> NVIQDLYLRELKDTKLAPSTLQD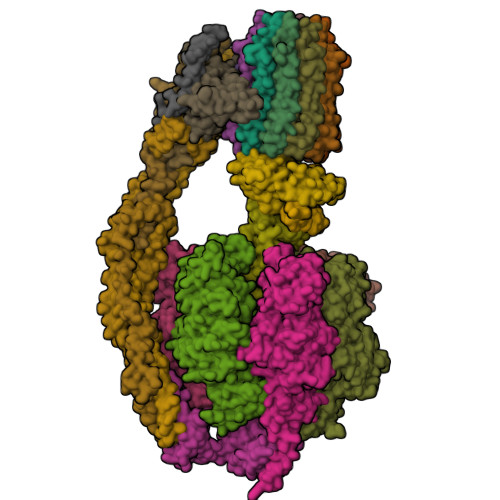AEGNVKPWNPPQKPNLPELELQGPEALKAYTEQNVETAHVAKESEEGESEPIEEDWLVLDDAEETKESH;> SLAKSAANKLDWAKVISSLRITGSTATQLSSFKKRNDEARRQLLELQSQPTEVDFSHYRSVLKNTSVIDKIESYVKQYKPVKIDASKQLQVIESFEKHAMTNAKETESLVSKELKDLQSTLDNIQSARPFDELTVDDLTKIKPEIDAKVEEMVKKGKWDVPGYKDRFGNLNVM;> MPQLVPFYFMNQLTYGFLLMITLLILFSQFFLPMILRLYVSRLFISKL;>[3x]ASTKAQPTEVSSILEERIKGVSDEANLNETGRVLAVGDGIARVFGLNNIQAEELVEFSSGVKGMALNLEPGQVGIVLFGSDRLVKEGELVKRTGNIVDVPVGPGLLGRVVDALGNPIDGKGPIDAAGRSRAQVKAPGILPRRSVHEPVQTGLKAVDALVPIGRGQRELIIGDRQTGKTAVALDTILNQKRWNNGSDESKKLYCVYVAVGQKRSTVAQLVQTLEQHDAMKYSIIVAATASEAAPLQYLAPFTAASIGEWFRDNGKHALIVYDDLSKQAVAYRQLSLLLRRPPGREAYPGDVFYLHSRLLERAAKLSEKEGSGSLTALPVIETQGGDVSAYIPTNVISITDGQIFLEAELFYKGIRPAINVGLSVSRVGSAAQVKALKQVAGSLKLFLAQYREVAAFAQFGSDLDASTKQTLVRGERLTQLLKQNQYSPLATEEQVPLIYAGVNGHLDGIELSRIGEFESSFLSYLKSNHNELLTEIREKGELSKELLASLKSATESFVATF;>[3x]ASAAQSTPITGKVTAVIGAIVDVHFEQSELPAILNALEIKTPQGKLVLEVAQHLGENTVRTIAMDGTEGLVRGEKVLDTGGPISVPVGRETLGRIINVIGEPIDERGPIKSKLRKPIHADPPSFAEQSTSAEILETGIKVVDLLAPYARGGKIGLFGGAGVGKTVFIQELINNIAKAHGGFSVFTGVGERTREGNDLYREMKETGVINLEGESKVALVFGQMNEPPGARARVALTGLTIAEYFRDEEGQDVLLFIDNIFRFTQAGSEVSALLGRIPSAVGYQPTLATDMGLLQERITTTKKGSVTSVQAVYVPADDLTDPAPATTFAHLDATTVLSRGISELGIYPAVDPLDSKSRLLDAAVVGQEHYDVASKVQETLQTYKSLQDIIAILGMDELSEQDKLTVERARKIQRFLSQPFAVAEVFTGIPGKLVRLKDTVASFKAVLEGKYDNIPEHAFYMVGGIEDVVAKAEKLAAEAN;> ATLKEVEMRLKSIKNIEKITKTMKIVASTRLSKAEKAKISAKKMDEAEQLFYKNAETKNLDVEATETGAPKELIVAITSDKGLCGSIHSQLAKAVRRHLNDQPNADIVTIGDKIKMQLLRTHPNNIKLSINGIGKDAPTFQESALIADKLLSVMKAGTYPKISIFYNDPVSSLSFEPSEKPIFNAKTIEQSPSFGKFEIDTDANVPRDLFEYTLANQMLTAMAQGYAAEISARRNAMDNASKNAGDMINRYSILYNRTRQAVITNELVDIITGASSLG;> AEAAAASSGLKLQFALPHETLYSGSEVTQVNLPAKSGRIGVLANHVPTVEQLLPGVVEVMEGSNSKKFFISGGFATVQPDSQLCVTAIEAFPLESFSQENIKNLLAEAKKNVSSSDAREAAEAAIQVEVLENLQSVLK;> SAWRKAGISYAAYLNVAAQAIRSSLKTELQTASVLNRSQTDAFYTQYKNGTAASEPTPITK;> MLKRFPTPILKVYWPFFVAGAAVYYGMSKAADLSSNT;>[10x]MQLVLAAKYIGAGISTIGLLGAGIGIAIVFAALINGVSRNPSIKDTVFPMAILGFALSEATGLFCLMVSFLLLFGV;> VSTLIPPKVVSSKNIGSAPNAKRIANVVHFYKSLPQGPAPAIKANTRLARYKAKYFDGDNASGKPLWHFALGIIAFGYSMEYYFHLRHHKGAEEH;> SPLDQFEIRTLFGLQSSFIDLSCLNLTTFSLYTIIVLLVITSLYTLTNNNNKIIGSRWLISQEAIYDTIMNMTKGQIGGKNWGLYFPMIFTLFMFIFIANLISMIPYSFALSAHLVFIISLSIVIWLGNTILGLYKHGWVFFSLFVPAGTPLPLVPLLVIIETLSYFARAISLGLRLGSNILAGHLLMVILAGLTFNFMLINLFTLVFGFVPLAMILAIMMLEFAIGIIQGYVWAILTASYLKDAVYLH;> ASKAAAPPPVRLFGVEGTYATALYQAAAKNSSIDAAFQSLQKVESTVKKNPKLGHLLLNPALSLKDRNSVIDAIVETHKNLDGYVVNLLKVLSENNRLGCFEKIASDFGVLNDAHNGLLKGTVTSAEPLDPKSFKRIEKALSASKLVGQGKSLKLENVVKPEIKGGLIVELGDKTVDLSISTKIQKLNKVLEDSI;> MSSTPEKQTDPKAKANSIINAIPGNNILTKTGVLGTSAAAVIYAISNELYVINDESILLLTFLGFTGLVAKYLAPAYKDFADARMKKVSDVLNASRNKHVEAVKDRIDSVSQLQNVAETTKVLFDVSKETVELESEAFELKQKVELAHEAKAVLDSWVRYEASLRQLEQRQLAKSVISRVQSELGNPKFQEKVLQQSISEIEQLLSKLK3-[(1~{R})-2-(~{tert}-butylamino)-1-[methanoyl-[[3,4,5-tris(fluoranyl)phenyl]methyl]amino]-2-oxidanylidene-ethyl]-6-chloranyl-1~{H}-indole-2-carboxylic acid | C23 H21 Cl F3 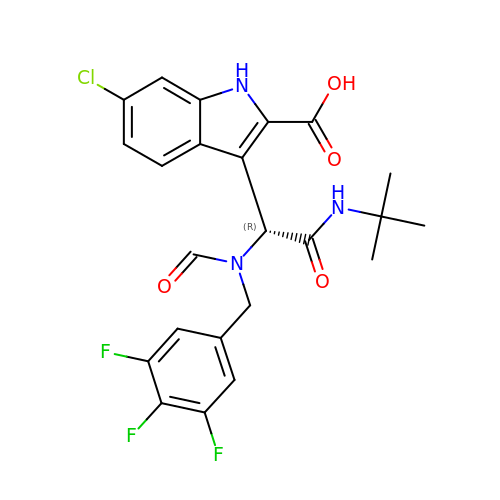N3 O4 | FZINKXKQKUDBDP-HXUWFJFHSA-N>CCGGACGAGGUGCGCCGUACCCGGUCAGGACAAGACGGCGC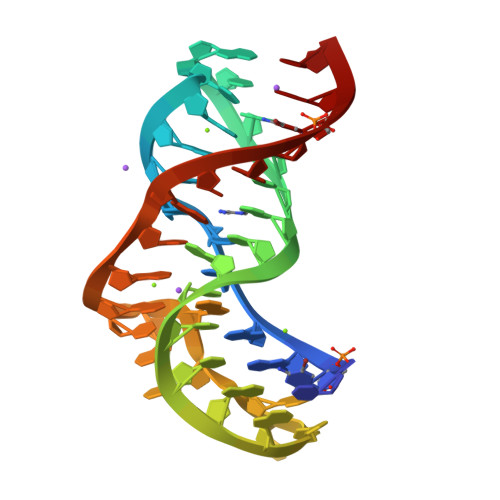[2x]> GLGDLIEGVVEGVTRNALTPLTPANNLPDTQSSGPAHSKEIPALTAVETGATNPLVPSDTVQTRHVIQKRTRSESTVESFFARGACVAIIEVDNDAPTKRASKLFSVWKITYKDTVQLRRKLEFFTYSRFDMELTFVVTSNYTDANNGHALNQVYQIMFIPPGAPIPGKWNDYTWQTSSNPSVFYTYGAPPARISVPYVGIANAYSHFYDGFAKVPLAGQASTEGDSLYGAASLNDFGSLAVRVVNDHNPTKLTSKIRVYMKPKHVRVWCPRPPRAVPYYGPGVDYKDGLAPLPEKGLTTY;> MGAQVSSQKVGAHENSNRAYGGSTINYTTINYYRDSASNAASKQDFAQDPSKFTEPIKDVLIKTAPTLNSPNIEACGYSDRVMQLTLGNSTITTQEAANSVVAYGRWPEYIKDSEANPVDQPTEPDVAACRFYTLDTVTWRKESRGWWWKLPDALKDMGLFGQNMFYHYLGRAGYTVHVQCNASKFHQGALGVFAVPEMCLAGDSTTHMFTKYENANPGEKGGEFKGSFTLDTNATNPARNFCPVDYLFGSGVLAGNAFVYPHQIINLRTNNCATLVLPYVNSLSIDSMTKHNNWGIAILPLAPLDFATESSTEIPITLTIAPMCCEFNGLRNITVPRTQ;> GLPVLNTPGSNQYLTADNYQSPCAIPEFDVTPPIDIPGEVRNMMELAEIDTMIPLNLTNQRKNTMDMYRVELNDAAHSDTPILCFSLSPASDPRLAHTMLGEILNYYTHWAGSLKFTFLFCGSMMATGKLLVSYAPPGAEAPKSRKEAMLGTHVIWDIGLQSSCTMVVPWISNTTYRLTINDSFTEGGYISMFYQTRVVVPLSTPRKMDILGFVSACNDFSVRLLRDTTHISQEAMPQ

Poliovirus (PV) is the causative agent of poliomyelitis, a highly infectious disease, which can cause paralysis and can be fatal. Mature PV virions are ~30 nm diameter icosahedral capsids comprising 60 copies of VP1-VP420. Empty capsids (ECs), which are also produced during infection, are antigenically indistinguishable from mature viral particles but do not contain viral genome and do not cleave VP022. ECs have potential as virus-like particle (VLP) vaccines to replace the current PV vaccines; however, recombinantly expressed wt ECs are inherently unstable and readily convert to an expanded form.

As yields of PV2-SC6b were lower than those of PV1-SC6b or PV3-SC8 we investigated shaker flask expression of an alternative stabilised PV2, termed PV2-SC5a27,42. PV2-SC5a produced more D Ag/100 mL than PV2-SC6b in both flask and bioreactor expression systems (threefold and ~2-fold respectively). PV2-SC5a was highly stable, with ~75% D Ag remaining at 50 °C and ~40% D Ag at 55 °C, outperforming both PV2-SC6b and BRP. Detailed structural analyses and comparison of the PV2-SC6b and PV2-SC5a VLPs from bioreactor production were performed by single particle cryo-EM. Data were collected as described in “Methods”. Data processing yielded a final set of 113,853 particles for PV2-SC6b and 147,409 particles for PV2-SC5a, and icosahedral reconstructions of 2.4 Å and 2.1 Å resolution, respectively. The structures confirm that both PV2 VLPs adopt a homogeneous D Ag conformation, with negligible or no particles observed in C Ag form. The quality of the cryo-EM electron potential maps is sufficient to resolve the stabilising mutations and confirm that they introduce no significant perturbations to the structure and do not impinge on the antigenic surface of the particle. Based on the extent of the observed electron potential map in the VP1 pockets of both PV2-SC6b and PV2-SC5a, a sphingosine lipid moiety of carbon length 18 was modelled into the maps. For PV2-SC6b the mutation in subunit VP4 I57V (I57V in VP0) and for PV2-SC5a the mutation in subunit VP1 T41I, were in disordered regions of the map and were not modelled. However, in the presence of adjuvant, the response to PV2-SC5a VLPs equalled the neutralising antibody titres elicited by IPV to 0.25 of a human dose, as observed previously for PV1-SC6b and PV3-SC8. Therefore, these data suggest that in the presence of a licensed adjuvant, PV2-SC5a VLPs are at least as immunogenic as IPV per D Ag.> MLREFSFYDVPPAHVPPVSEPLEIACYSLSRDRELLLDDSKLSYYYPPPLFSDLNTGFPNRFHPPKSDPDPIS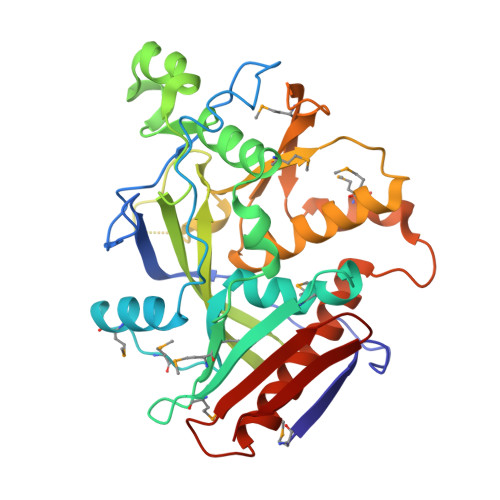IVKDVLMTKGIQMNSSFLTWRGLITKIMCAPLDPRNHWETYLVMDPTSGIIMMEERTRSETSYANQDRMCYWGYKFEAISTLPEIWDACSRDQIEQRDNQDVVPDEQYCSIVKINIGKSKLILAGEVDCIWDKKPCSAKESDVHSDDGTIEEDASNAENPNLHYVELKTSKKYPLENYGMRKKLLKYWAQSFLLGIGRIIIGFRDDNGILIEMKELFTHQIPKMLRPYFKPNDWTPNRLLVVLEHALEWIKQTVKQHPPSTEFTLSYTGGSKLVLRQII>[2x]FTETTIVVH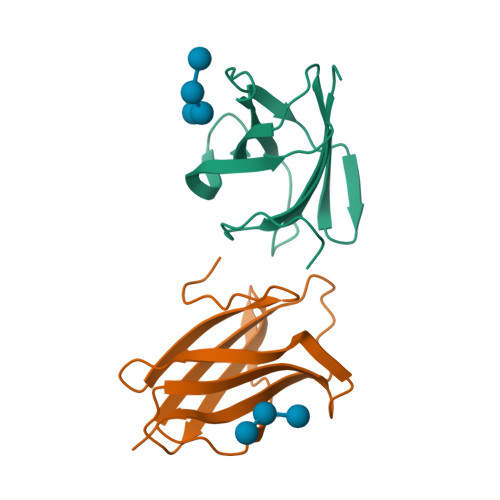YHRYDGKYDGWNLWIWPVEPVSQEGKAYQFTGEDDFGKVAVVKLPMDLTKVGIIVRLNEWQAKDVAKDRFIEIKDGKAEVWILQGVEEIFYEKP>MAHHHHHHVGTMLTIYSDDHHLHHGSCELIDGKLMPCFEMPKRADHILQRVKDRNIGEIREPQDFGRDPIQRIHTAEYLNFFEGAWARWQEQDGTGDLLPYTWPARTLSQRLPTSLHGQLGYYSFDAGAPITAGTWQAAYSAAQVALTAQHEITNGAHSAFALCRPPGHHAASDVMGGYCYLNNAAIAAQAFIDQGHKRVAILDVDYHHGNGTQSIFYSRSDVLFTSIHGDPKFEFPFFLGHADEHGEGTGEGFNINYPLPAGSAWDSWGAALDDACKRINAFDAEVVIVSLGVDTYKEDPISQFKLDSPDYLSMGERIAAMGLPTLFVMEGGYAVEAIGVNAVNVLEGFENV[2x]

Classical Zn2+-dependent deac(et)ylases play fundamental regulatory roles in life and are well characterized in eukaryotes regarding their structures, substrates and physiological roles. Structurally, these enzymes are composed of a central eight-stranded parallel β-sheet flanked by α-helices on each site, known as the α/β-arginase/deacetylase fold. All active site residues were conserved, as shown by the multiple sequence alignment and the structural alignment, suggesting a general acid/base catalytic mechanism for the bacterial enzymes as described for the eukaryotic counterparts. These enzymes mediate catalysis using a penta-coordinated catalytic Zn2+ ion coordinated by two aspartates and a histidine (KpHdaH (1b): Asp181, Asp269, His183).

To explain the molecular basis for classical deacylases to act as polyamine deacetylases, we structurally characterized the enzyme PsApaH. The crystal structure of PsApaH confirmed the analytical SEC experiments supporting cluster 4 enzymes forming head-to-head dimers. Dimer formation is mediated by a structural feature distinct to polyamine deacetylases, i.e. L2-loop (PSL: polyamine-specificity loop). An important specificity-determining interaction is a salt bridge between R95 of the L2-loop of one monomer and D163 of the other monomer of the dimer. The N-terminal L1-loop interacts in trans with the L2-loop, occluding the active site and thereby restricting the access of acetylated peptides. This L1-loop is highly flexible in the apo form, as it was not resolved in our apo structure of PsApaH. In our PsApaH structure, Y168 exists in two alternative conformations supporting the flexibility in the unliganded state. In PsApaH, this Glu106 is replaced by His106 explaining the higher acetylpolyamine substrate promiscuity for PsApaH. PsApaH and the P. aeruginosa enzymes PA1409 and PA0321 also contain the PIS-motif, which explains the higher level of promiscuity observed for bacterial polyamine deacetylases. Notably, the bacterial polyamine deacetylases also contain a conserved RPP-motif (PsApaH (4)/M. ramosa ApaH: 154-RPPGHH-159) and an XGGY-motif (PsApaH (4)/M. ramosa ApaH: 320-EGGY−323), identified for robust deacetylases such as KpHdaH (1b) but not present in deacylases with activity for longer acyl-chains, suggesting these enzymes prefer to remove acetyl-groups from polyamines but no longer acyl-chains. Only the cluster 4 enzyme ApaH from Pseudomonas sp., PsApaH, showed activity as polyamine deacetylase.> MVEATAQETDRPRFSFSIAAREGKARTGTIEMKRGVIRTPAFMPVGTAATVKALKPETVRATGADIILGNTYHLMLRPGAERIAKLGGLHSFMGWDRPILTDSGGFQVMSLSSLTKQSEEGVTFKSHLDGSRHMLSPERSIEIQHLLGSDIVMAFDECTPYPATPSRAASSMERSMRWAKRSRDAFDSRKEQAENAALFGIQQGSVFENLRQQSADALAEIGFDGYAVGGLAGGEGQDEMFRVLDFSVPMLPDDKPHYLMGVGKPDDIVGAVERGIDMFDCVLPTRSGRNGQAFTWDGPINIRNARFSEDLKPLDSECHCAVCQKWSRAYIHHLIRAGEILGAMLMTEHNIAFYQQLMQKIRDSISEGRFSQFAQDFRARYFARNS

Transfer RNA–guanine transglycosylase (Tgt, EC 2.4.2.29) catalyses the exchange of a specific guanine base in tRNA molecules by a substituted 7-deazaguanine. Bacterial Tgt functions as a homodimer in which the protomer consists of a (βα)8 barrel harbouring a Zn2+ binding subdomain close to the C-terminus. The reaction follows a ping-pong mechanism including a covalent Tgt⋅tRNA intermediate. Hence, in an attempt to generate a model system for the active site of human Tgt and to gain insights into the relevance of particular amino acids for substrate base selectivity, we adapted the Z. mobilis Tgt active site by site-directed mutagenesis in order to mimic that of the human enzyme.

In order to investigate the importance of Gly232 and Val161 in human Tgt for queuine recognition, we created a doubly mutated variant of the Z. mobilis enzyme in which the corresponding Val233 and Cys158 were exchanged by glycine and valine, respectively. In addition, we created two further variants, each containing solely one of the above-mentioned amino acid exchanges. To allow the interpretation of the obtained data at a structural level, we determined the crystal structures of the mutated Tgt variants created in this study in their apo-forms as well as in complex with preQ1 and queuine. The replacement of Val233 by glycine results in a considerable gain of space in the substrate binding pocket most probably required for the accommodation of the dihydroxy-cyclopentenyl moiety of queuine. In contrast, under the same conditions a faint band representing the covalent enzyme·tRNA complex was observed for Tgt(Val233Gly) and Tgt(Cys158Val/Val233Gly) indicating that the reinsertion rate of the excised guanine was significantly decreased with these Tgt variants (lanes 5 and 11).>[3x]ATAAEIAALPRQKVELVDPPFVHAHSQVAEGGPKVVEFTMVIEEKKIVIDDAGTEVHAMAFNGTVPGPLMVVHQDDYLELTLINPETNTLMHNIDFHAATGALG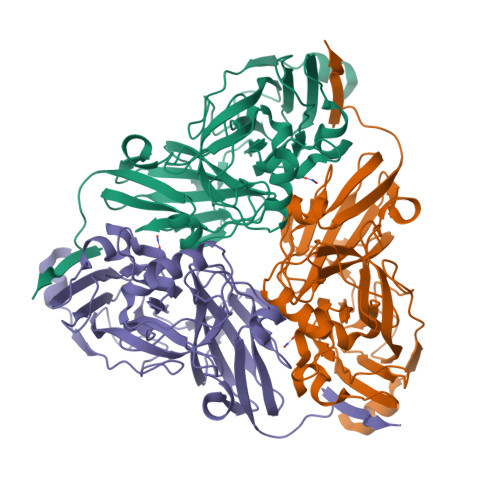GGGLTEINPGEKTILRFKATKPGVFVYHCAPPGMVPWHVVSGMNGAIMVLPREGLHDGKGKALTYDKIYYVGEQDFYVPRDENGKYKKYEAPGDAYEDTVKVMRTLTPTHVVFNGAVGALTGDKAMTAAVGEKVLIVHSQANRDTRPHLAGGHGDYVWATGKFNTPPDVDQETWFIPGGAAGAAFYTFQQPGIYAYVNHNLIEAFELGAAAHFKVTGEWNDDLMTSVLAPSGTIEGR>[4x]ALESAQESHALHHQNAAALRFQFHITREQAREIVKLCPNCPDWGHAPQLGVNPRGLKPRVLWQMDVTHVSEFGKLKYVHVTVDTYSHFTFATARTGEATKDVLQHLAQSFAYMGIPQKIKTDNAPAYVSRSIQEFLARWKISHVTGIPYNPQGQAIVERTHQNIKAQLNKLQKAGKYYTPHHLLAHALF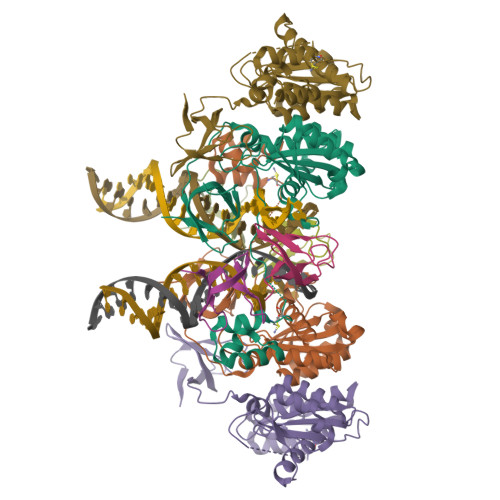VLNHVNMDNQGHTAAERHWGPISADPKPMVMWKDLLTGSWKGPDVLITAGRGYACVFPQDAESPIWVPDRFIRPFT;>[4x]PMVMWKDLLTGSWKGPDVLITAGRGYACVFPQDAESPIWVPDRFIRPFT> MATLKRDKGLDNTLKVLKQGYLYTTNQRNRLNTSVFQTKALGGKPFVVVTGKEGAEMFYNNDVVQREGMLPKRIVNTLFGKGAIQTVDGKKHVDRKALFMSLMTEGNLNYVRELTRTLWHANTQRMESMDEVNIYRESIVLLTKVGTRWAGVQAPPEDIERIATDMDIMIDSFRALGGAFKGYKASKEARRRVEDWLEEQIIETR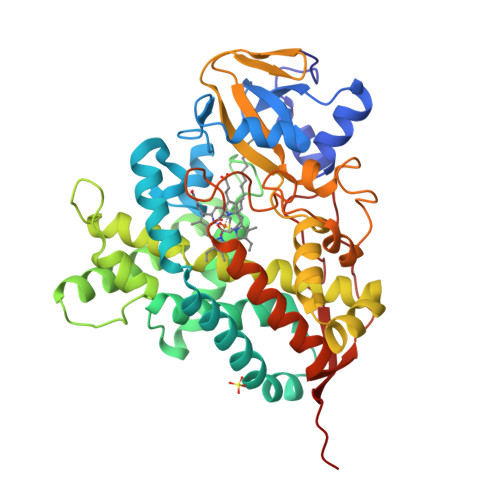KGNIHPPEGTALYEFAHWEDYLGNPMDSRTCAIDLMNTFRPLIAINRFVSFGLHAMNENPITREKIKSEPDYAYKFAQEVRRYYPFVPFLPGKAKVDIDFQGVTIPAGVGLALDVYGTTHDESLWDDPNEFRPERFETWDGSPFDLIPQGGGDYWTNHRCAGEWITVIIMEETMKYFAEKITYDVPEQDLEVDLNSIPGYVKSGFVIKNVREVVDRT;> HHHHHHMATLKRDKGLDNTLKVLKQGYLYTTNQRNRLNTSVFQTKALGGKPFVVVTGKEGAEMFYNNDVVQREGMLPKRIVNTLFGKGAIQTVDGKKHVDRKALFMSLMTEGNLNYVRELTRTLWHANTQRMESMDEVNIYRESIVLLTKVGTRWAGVQAPPEDIERIATDMDIMIDSFRALGGAFKGYKASKEARRRVEDWLEEQIIETRKGNIHPPEGTALYEFAHWEDYLGNPMDSRTCAIDLMNTFRPLIAINRFVSFGLHAMNENPITREKIKSEPDYAYKFAQEVRRYYPFVPFLPGKAKVDIDFQGVTIPAGVGLALDVYGTTHDESLWDDPNEFRPERFETWDGSPFDLIPQGGGDYWTNHRCAGEWITVIIMEETMKYFAEKITYDVPEQDLEVDLNSIPGYVKSGFVIKNVREVVDRT PUF proteins, named for PUM (Pumilio) and FBF (fem-3 binding factor), are an exemplary system for understanding the divergence of RNA recognition within eukaryotic RNA-binding protein families. Eight PUM repeats are arranged in a crescent shape with the RNA bound on the concave face of the protein. Each repeat contributes a trio of amino acid residues, termed a tripartite recognition motif (TRM), that directly contact the opposing RNA base. FBF recognizes a 9-nt motif, 5´-UGURNNAUA-3´, whereas PUF-8 binds an 8-nt sequence, 5´-UGUANAUA-3´.

To clarify the molecular basis of this divergent binding specificity, we determined a 2.6 Å crystal structure of PUF-8 bound to an 8-nt PBE RNA, 5´-UGUAUAUA-3´. The overall structure of the RNA-binding domain of PUF-8 is similar to that of other classical PUF proteins with eight α-helical PUM repeats (R1 to R8) and flanking regions at both the N- and C-termini (R1´ and R8´). PUM repeats R8-R5 bind to the 5´-UGUA sequence, and PUM repeats R3-R1 bind to bases 6–8, the AUA-3´ sequence. The 5´-UGUA and AUA-3´ base specific interactions bracket a central region in which the 5th base turns away from the concave RNA-binding surface and stacks directly with the 4th base. As a result, the 5th base is not recognized by PUF-8, and PBE RNAs with any nucleotide at position 5 are bound by PUF-8 with similar affinity. R362 in R5 is located at the position that typically would form stacking interactions between the 4th and 5th RNA bases, but instead the side chain is moved aside. This type of recognition was observed in crystal structures of human PUM1 and PUM2 with some RNA sequences and is termed the base-omission mode. The mode of RNA recognition and overall curvature of PUF-8 are reminiscent of the one repeat to one base modularity of PUM1. Superposition of the structures highlights this relationship as the RMSD is 1.2 Å over 293 Cα atoms, and the inner RNA-binding helices align with similar curvature. Aligning repeats R5-R8 illustrates that the curvature of the PUF-8 scaffold contrasts starkly with the flatter FBF-2 scaffold.

>[3x]GTTTDDLLTRYRANPAMMKNLKLSDIRGALLKFAKDQVGSRFIQQELASSKDRFEKDSIFDEVVSNADELVDDIFGNYVVQKFFEYGEERHWARLVDAIIDRVPEYAFQMYACRVLQKALEKINEPLQIKILSQIRHVIHRCMKDQNGNHVVQKAIEKVSPQYVQFIVDTLLESSNTIYEMSVDPYGCRVVQRCLEHCSPSQTKPVIGQIHKRFDEIANNQYGNYVVQHVIEHGSEEDRMVIVTRVSNNLFEFATHKYSSNVIEKCLEQGAVYHKSMIVGAACHHQEGSVPIVVQMMKDQYANYVVQKMFDQVTSEQRRELILTVRPHIPVLRQFPHGKHILAKLEKYFQKPAVMS>[2x]MVLYFIGLGLYDERDITVKGLEIAKKCDYVFAEFYTSLMAGTTLGRIQKLIGKEIRVLSREDVELNFENIVLPLAKENDVAFLTPGDPLVATTHAELRIRAKRAGVESYVIHAPSIYSAVGITGLHIYKFGKSATVAYPEGNWFPTSYYDVIKENAERGLHTLLFLDIKAEKRMYMTANEAMELLLKVEDMKKGGVFTDDTLVVVLARAGSLNPTIRAGYVKDLIREDFGDPPHILIVPGKLHIVEAEY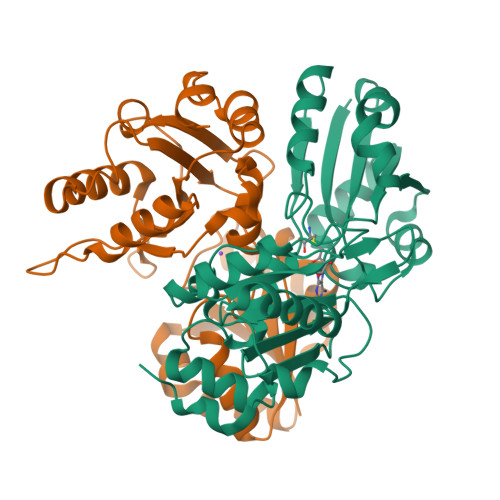LVEMAGAPREILRVNV>TYLDRLALRYDREGEPSQLAAVDIFVSTVDPLKEPPLVTANTVLSILAVDYPVDKVSCYVSDDGAAMLSFESLAETSEFARKWVPFCKKYSIEPRAPEWYFAAKIDYLKDKVQTSFVKDRRAMKREYEEFKIRINALVSKALKCPEEGWVMQDGTPWPGNNTRDHPGMIQVFLGQNGGLDAEGNELPRLVYVSREKRPGFQHHKKAGAMNALVRVSAVLTNGPFILNLDCDHYINNSKALREAMCFLMDPNLGKQVCYVQFPQRFDGIDKNDRYANRNTVFFDINLRGLDGIQGPVYVGTGCVFNRTALYGYEPGSGSGSLEKRFGQSAVFVASTLMENGGVPPSATPENLLKEAIHVISCGYEDKSDWGMEIG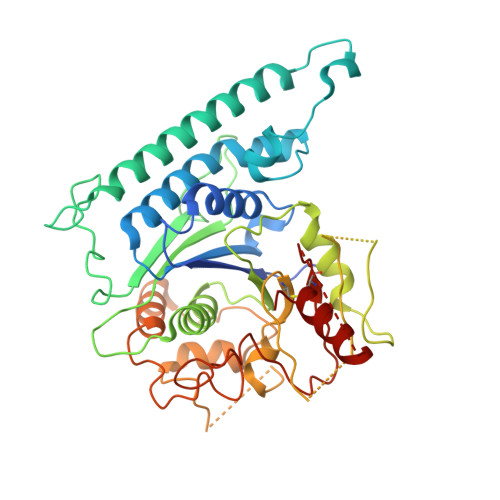WIYGSVTEDILTGFKMHARGWRSIYCMPKLPAFKGSAPINLSDRLNQVLRWALGS[2x]> DFQSESYKDAYSRINAIVIEGEQEAFDNYNRLAEMLPDQRDELHKLAKMEQRHMKGFMACGKNLSVTPDMGFAQKFFERLHENFKAAAAEGKVVTCLLIQSLIIECFAIAAYNIYIPVADAFARKITEGVVRDEYLHRNFGEEWLKANFDASKAELEEANRQNLPLVWLMLNEVADDARELGMERESLVEDFMIAYGEALENIGFTTREIMRMSAYGLAAV;> LDFQSESYKDAYSRINAIVIEGEQEAFDNYNRLAEMLPDQRDELHKLAKMEQRHMKGFMACGKNLSVTPDMGFAQKFFERLHENFKAAAAEGKVVTCLLIQSLIIECFAIAAYNIYIPVADAFARKITEGVVRDEYLHRNFG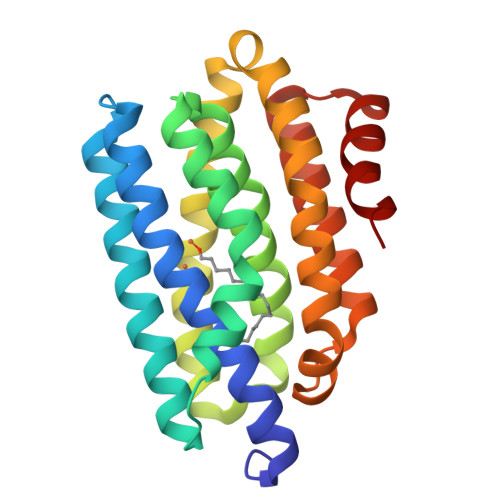EEWLKANFDASKAELEEANRQNLPLVWLMLNEVADDARELGMERESLVEDFMIAYGEALENIGFTTREIMRMSAYGLAAV>XEVKQLEAEVEEIESEVWHLENEVARLEKENAECEA[3x];>[3x]XKVKQL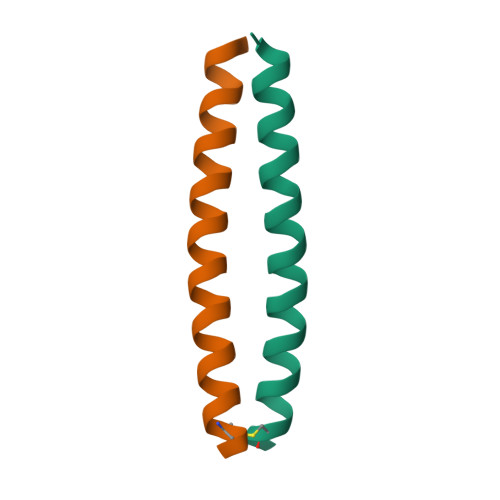KAKVEELKSKLWHLKNKVARLKKKNAECKA> 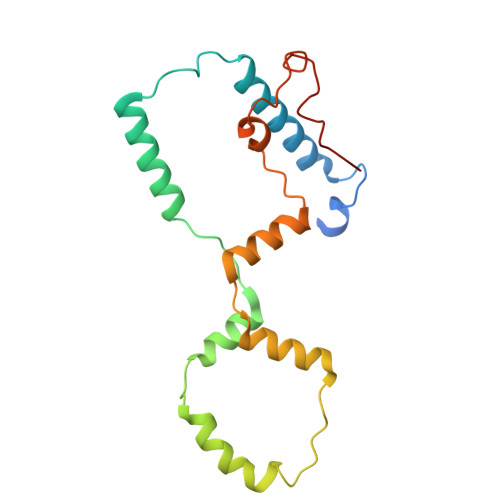MRRKTTLNIGQVICFSSWNDGSEGYEWKSRALSEKRSLALEFLGNVNKRVSIHDAIRLKADINKKAISNVSCPSFFSGIEGADEDEDQSDMSLCSLLGVLEGEIETDCITHLSPSDASLLKEEFLCDYDPSDTKRMAKWVNLRSETSDYQSYGAIPEGERSLWSAWYLRNIKAGKKPI> GMHSAALLQKVDELPRLPKAIAE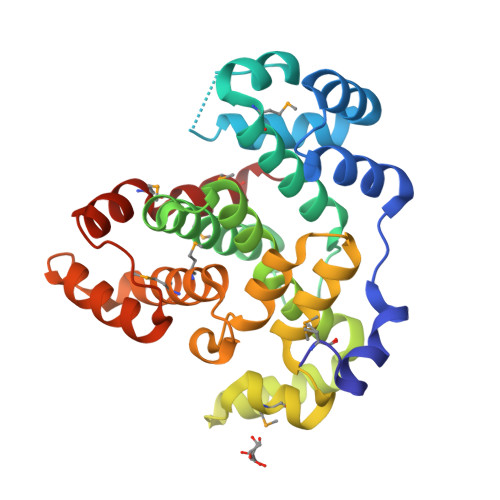LLDVVNNEDSTVKAVSEKLSHDPVLSARVLRLANSARFGCSREVGTIDDAVVRLGMQTLRTLVIASAVVGAVPKVEGFDLADFWGNTFEVAIICQELAKRLGTLPEEAFTCGILHSIGELLIVNGDPAVAATISAAVADGADRNLMEKELLGYDNAEIGALLAQSWKFTPHLVKGIQFQNHPKSAEPYSKLAGMLAMAKQIAADWDKIPDDERTSWLAQINILAGIKVDLGGLAEKLAKMHGQGMEMGKQLA>[2x]MKHHHHHHPMPKKIVVFSLAEEL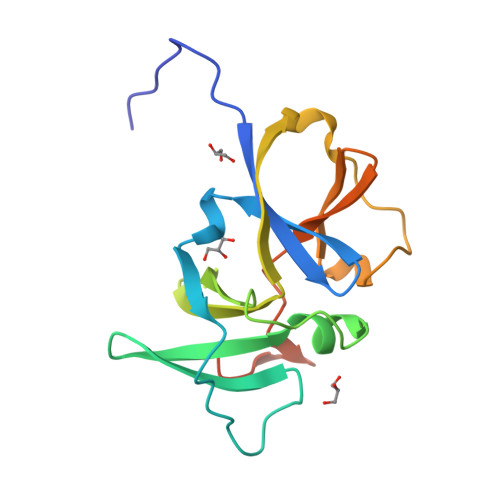YGLDIFDVHEVVKDVSITKIPETPEFIEGIINLRGKIIPVIDLKKRFGIGKRGKSKDSRIIIVEILGQKAGLIVDAVHEVIPIDENSIEPPPPVTTIDTAFVEGIAKTDDKMIIIIKLHFLFEVNGKEMLLNTSSEGTKERS>SIVIASAARTAVGSFNGAFANTPAHELGATVISAVLERAGVAAGEVNEVILGQVLPAGEGQNPARQAAMKAGVPQEATAWGMNQLCGSGLRAVALGMQQIATGDASIIVAGGMESMSMAPHCAHLRGGVKMGDFKMIDTMIKDGLTDAFYGYHMGTTAENVAKQWQLSRDEQDAFAVASQNKAEAAQKDGRFKDEIVPFIVKGRKGDITVDADEYIRHGATLDSMAKLRPAFDKEGTVTAGNASGLNDGAAAALLMSEAEASRRGIQPLGRIVSWATVGVDPKVMGTGPIPASRKALERAGWKIGDLDLVEANEAFAAQACAVNKDLGWDPSIVNVNGGAIAIGHPIGASGARILN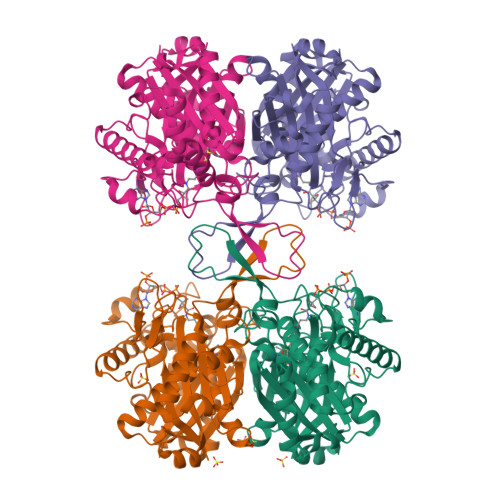TLLFEMKRRGARKGLATLCIGGGMGVAMCIESL[4x]>MSSASSNARDEVIAAIHEEADWVDRTVYPFESRCIGLSSGAVHYIDEGPDDGGRETLLMLHGNPTWSFLYRHLVRDLRDEYRCVALDYLGFGLSERPTDFSYRPEDHADVVEEFIDELGLEDVVLVGHDWGGPIGFSYAIDHPENVGGLVVMNTWMWPVSDDKHFSRFSKLLGGRIGRELCERYDLFTRVIMPMGFADRSRFTESA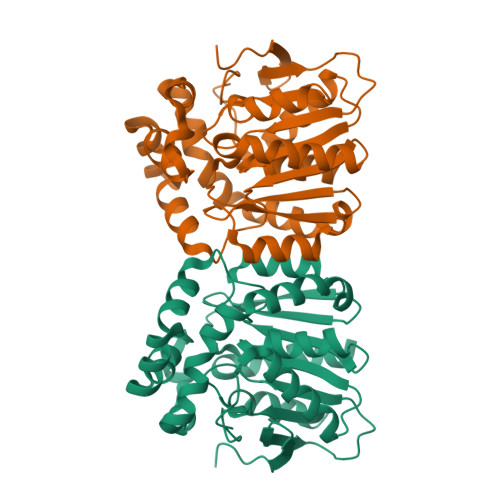REQYRAANRGDRTGTGIFPQAILGSRAWLSSLWEQRDNIADIPARIIWGMEDSAFRPAELRTFEALFEDSSTVRLYGVGHYVPEEFGSDLVPLVREFLEEVLEVLFQ[2x]>[2x]MLLYMRFTENFERAKKEALMSLEIALRKGEVDEDIIPLLKKINSIENYFTTSSCSGRISVMEMPHFGDKVNAKWLGKWHREVSLYEVLEAIKK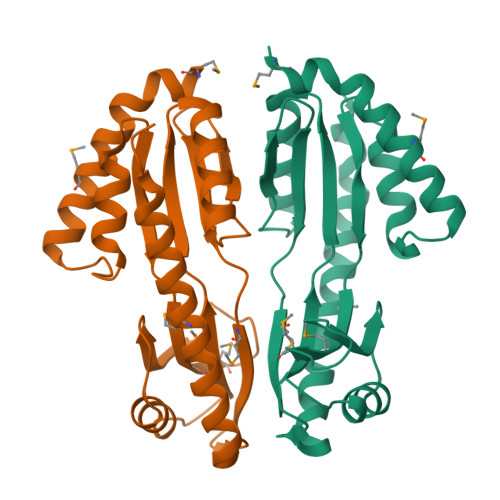HRSGQLWFLVRSPILHVGAKTLEDAVKLVNLAVSCGFKYSNIKSISNKKLIVEIRSTERMDVLLGENGEIFVGEEYLNKIVEIANDQMRRFKEKLKRLESKINALNR> HHHHHHHHHHENLYFQGGGSMEVEQTSVRSDTNSTCEYLDAEGDPESPNLYQEADPDQEAEQQNHSIISELRDGLGTMRDNSALSPEPGQENKGLAASVESLALSTSTSAKTEDSIGGGLEEEYDYQHDSLWQGQKKHIFILSEAGKPIFSLHGNEDKLATLFGVIQALVSFVQMGQDAITSIHAGGIKFAFMQRSSLILVAASRSNMSVQQLQLQLGDVYNQILSILTYSHMTKIFERRKNFDLRRLLSGSERLFYNLLANDSSSAKVSNNIFTFLTNSIRVFPLPTTIRSQITSAIQSNCSKIKNLVFAVLIANNKLIALVRMKKYSIHPADLRLIFNLVECSESFKSSENWSPICLPKFDMNGYLHAHVSYLADDCQACLLLLSVDRDAFFTLAEAKAKITEKLRKSHCLEAINEELQQPFNAKLYQQVVGIPELRHFL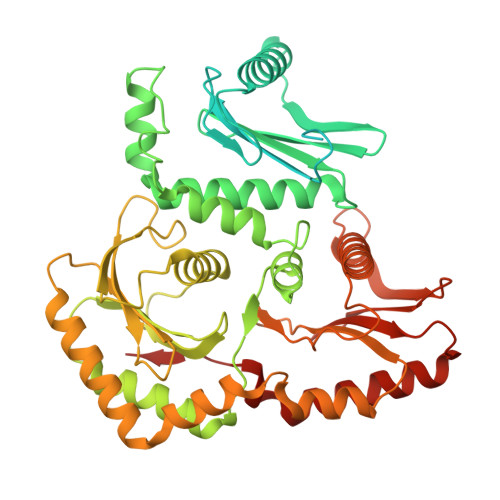YKPKSTAQLLCPMLRHPYKSLTELERLEAIYCDLLHRIHNSSRPLKLIYEMKEREVVLAWATGTYELYAIFEPVVDKATVIKYVDKLIKWIEKEYDVYFIRNHATF>MDYKFWYTQPVPKINDEFNE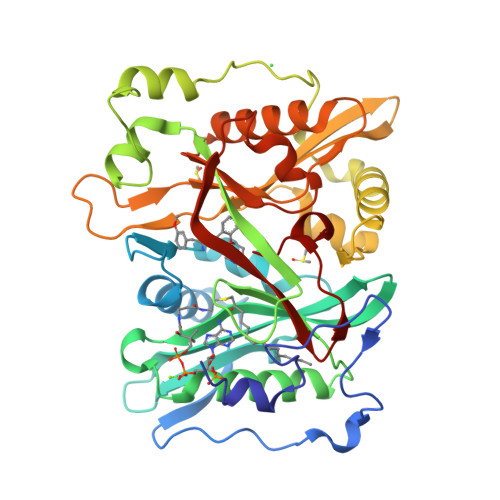SVNEPFISDNKVEDVRKDEYKLPPGYSWYVCDVKDEKDRSEIYTLLTDNYVEDDDNIFRFNYSAEFLLWALTSPNYLKTWHIGVKYDASNKLIGFISAIPTDICIHKRTIKMAEVNFLCVHKTLRSKRLAPVLIKEITRRINLENIWQAIYTAGVYLPKPVSDARYYHRSINVKKLIEIGFSSLNSRLTMSRAIKLYRVEDTLNIKNMRLMKKKDVEGVHKLLGSYLEQFNLYAVFTKEEIAHWFLPIENVIYTYVNEENGKIKDMISFYSLPSQILGNDKYSTLNAAYSFYNVTTTATFKQLMQDAILLAKRNNFDVFNALEVMQNKSVFEDLKFGEGDGSLKYYLYNWKCASFAPAHVGIVLL[3x]> MEGSGEQPGPQPQHPGDHRIRDGDFVVLKREDVFKAVQVQRRKKVTFEKQWFYLDNVIGHSYGTAFEVTSGGSLQPKKKREEPTAETKEAGTDNRNIVDDGKSQKLTQDDIKALKDKGIKGEEIVQQLIENSTTFRDKTEFAQDKYIKKKKKKYEAIITVVKPSTRILSIMYYAREPGKINHMRYDTLAQMLTLGNIRAGNKMIVMETCAGLVLGAMMERMGGFGSIIQLYPGGGPVRAATACFGFPKSFLSGLYEFPLNKVDSLLHGTFSAKMLSSEPKDSALVEESNGTLEEKQASEQENEDSMAEAPESNHPEDQETMETISQDPEHKGPKERGSKKDYIQEKQRRQEEQRKRHLEAAALLSERNADGLIVASRFHPTPLLLSLLDFVAPSRPFVVYCQYKEPLLECYTKLRERGGVINLRLSET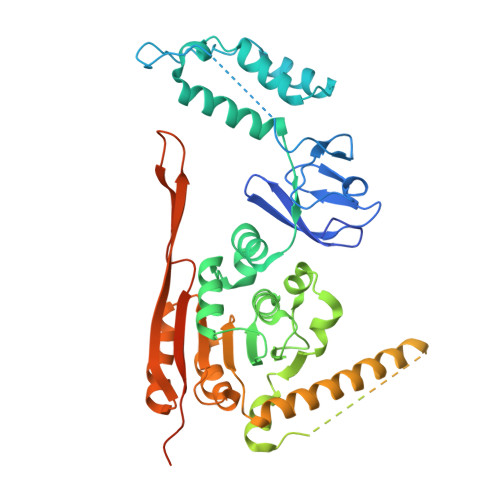WLRNYQVLPDRSHPKLLMSGGGGYLLSGFTVAMDNLKADTSLKSNASTLESHETEEPAAKKRKCPESDS> MGHHHHHHGSSIETDRVSKEFIEFLKTFHKTGQEIYKQTKLFLEGMHYKRDLSIEEQSECAQDFYHNVAERMQTRGKVPPERVEKIMDQIEKYIMTRLYKYVFCPETTDDEK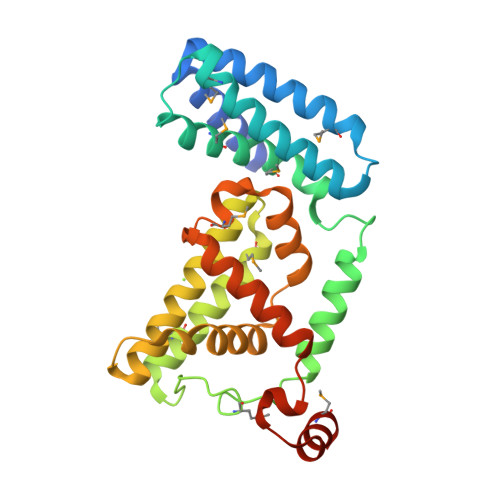KDLAIQKRIRALRWVTPQMLCVPVNEDIPEVSDMVVKAITDIIEMDSKRVPRDKLACITKCSKHIFNAIKITKNEPASADDFLPTLIYIVLKGNPPRLQSNIQYITRFCNPSRLMTGEDGYYFTNLCCAVAFIEKLDAQSLNLSQEDFDRYMSGQTSPRKQ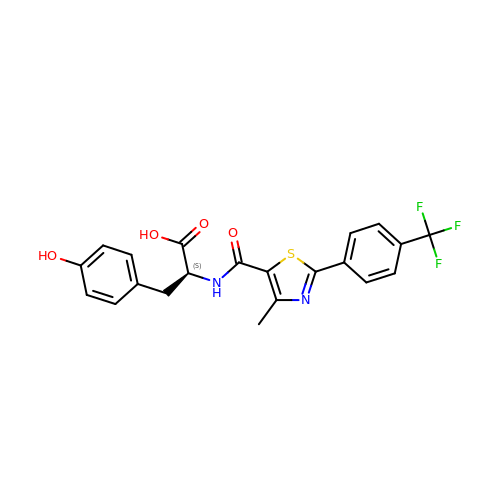N-({4-methyl-2-[4-(trifluoromethyl)phenyl]-1,3-thiazol-5-yl}carbonyl)-L-tyrosine | C21 H17 F3 N2 O4 S | VRYKCDADDIVMLC-INIZCTEOSA-N> SNASAAEAPLPQLRAYTVDASWLQPMAPLQVADHTWQIGTEDLTALLVQTAEGAVLLDGGMPQMAGHLLDNMKLRGVAPQDLRLILLSHAHADHAGPVAELKRRTGAHVAANAETAVLLARGGSNDLHFGDGITYPPASADRIIMDGEVVTVGGIAFTAHFMPG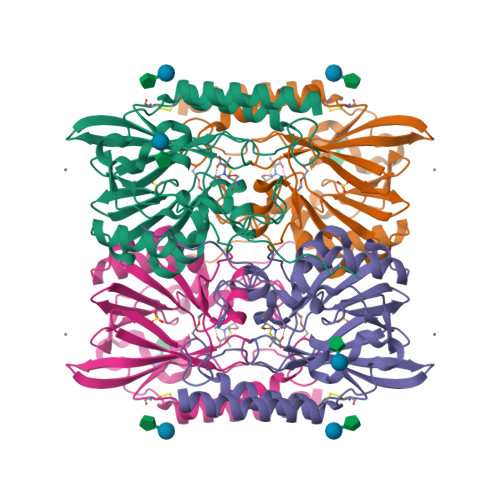HTPGSTAWTWTDTRDGKPVRIAYADSLSAPGYQLKGNPRYPRLIEDYKRSFATVRALPCDLLLTPHPGASNWNYAVGSKASAEALTCNAYADAAEKKFDAQLARETAGTR The nap particle is an immunogenic surface adhesion complex from Mycoplasma genitalium. It is essential for motility and responsible for binding sialylated oligosaccharides on the surface of the host cell. Cryo-electron tomography (cryo-ET) of M. genitalium revealed the tetrameric organization of the nap particle complex, consisting of two P140-P110 heterodimers. The P140-P110 heterodimers form the ‘tight interface’, while the ‘loose interface’ is formed between the two heterodimers.

In contrast to previous studies, this analysis by classification of the native nap particle displayed both the ‘open’ and the ‘closed’ state of the tight interface, resolved at 17 Å and 18 Å, respectively. Although the resolution obtained is insufficient to resolve the sialylated oligosaccharides in the crown region, the fact that we obtain classes with the ‘open’ conformation is conclusive evidence for the bound state. The resulting structure of the P110-P140 interaction site in the crown region for the ‘open’ state shows that the distance between P110 and P140 at the tight interface is sufficiently large so that the interfering loop (P140 residues 807–827) no longer interferes with the β-hairpin of P110 (residues 455–465). The structure indicates that P140 may additionally stabilize the binding to sialylated oligosaccharides by forming hydrogen bonds with residues from region 631–634 and loop 870–877 of P140, such as those between residues N634, S871 and 6′-SL. The binding of 6′-SL is stabilized by hydrogen bonds from both P110 and P140. Importantly, the opening and closing of the tight interface is accompanied by an interaction between P110 and P140 at the loose interface of the nap particle. In the ‘closed’ conformation, there is no density seen at the loose interface, whereas in the ‘open’ conformation, P110 and P140 come into proximity at the loose interface, thus indicating an interaction between loop 662–666 of P110 and loop 1173–1179 of P140. In fact, classes showing an opening and closing of the tight interface are always associated with a repositioning of the P110 stalk. In the open state, nap particle is bound to sialylated oligosaccharides mediated by P110 and further stabilized by P140. In addition, there is an interaction between P110 and P140 at the loose interface.

> MKTMRKQIYKKAYWLLLPFLPLALANTFLVKEDSKNVTAYTPFATPITDSKSDLVSLAQLDSSYQIADQTIHNTNLFVLFKSRDVKVKYESSGSNNISFDSTSQGEKPSYVVEFTNSTNIGIKWTMVKKYQLDVPNVSSDMNQVLKNLILEQPLTKYTLNSSLAKEKGKTQREVHLGSGQANQWTSQRNQHDLNNNPSPNASTGFKLTTGNAYRKLSESWPIYEPIDGTKQGKGKDSSGWSSTEENEAKNDAPSVSGGGSSSGTFNKYLNTKQALESIGILFDDQTPRNVITQLYYASTSKLAVTNNHIVVMGNSFLPSMWYWVVERSAQENASNKPTWFANTNLDWGEDKQKQFVENQLGYKETTSTNSHNFHSKSFTQPAYLISGIDSVNDQIIFSGFKAGSVGYDSSSSSSSSSSSSTKDQALAWSTTTSLDSKTGYKDLVTNDTGLNGPINGSFSIQDTFSFVVPYSGNHTNNGTTGPIKTAYPVKKDQKSTVKINSLINATPLNSYGDEGIGVFDALGLNYNFKSNQERLPSRTDQIFVYGIVSPNELRSAKSSADSTGSDTKVNWSNTQSRYLPVPYNYSEGIIDADGFKRPENRGASVTTFSGLKSIAPDGFANSIANFSVGLKAGIDPNPVMSGKKANYGAVVLTRGGVVRLNFNPGNDSLLSTTDNNIAPISFSFTPFTAAESAVDLTTFKEVTYNQESGLWSYIFDSSLKPSHDGKQTPVTDNMGFSVITVSRTGIELNQDQATTTLDVAPSALAVQSGIQSTTQTLTGVLPLSEEFSAVIAKDSDQNKIDIYKNNNGLFEIDTQLSNSVATNNGGLAPSYTENRVDAWGKVEFADNSVLQARNLVDKTVDEIINTPEILNSFFRFTPAFEDQKATLVATKQSDTSLSVSPRIQFLDGNFYDLNSTIAGVPLNIGFPSRVFAGFAALPAWVIPVSVGSSVGILFILLVLGLGIGIPMYRVRKLQDASFVNVFKKVDTLTTAVGSVYKKIITQTGVVKKAPSALKAANPSVKKPAAFLKPPVQPPSKPEGEQKAVEVKSEETKS;> MHQPKKRLAKKSWAFLTAALTLGVITGVGGYFLFNQNKQRSSVSNFAYQPKQLSVKHQQAVDETLTPWTWNNNNFSSLKITGENPGSFGLVRSQNDNLNISSVTKNSSDDNLKYLNAVEKYLDGQQNFAIRRYDNNGRALYDINLAKMENPSTVQRGLNGEPIFDPFKGFGLTGNAPTDWNEIKGKVPVEVVQSPHSPNLYFVLLVPKVALEYHNLNNQVVKESLEVKATQSSFNPTQRLQKDSPVKDSSKQGEKLSETTASSMSSGMATSTRAKALKVEVERGSQSDSLLKNDFAKKPLKHKNSSGEVKLEAEKEFTEAWKPLLTTDQIAREKGMGATVVSFYDAPYSENHTAFGLVDHIDPKKMVENYPPSWKTPKWNHHGIWDYNARNLLLQTTGFFNPRRHPEWFDEGQAKADNTSPGFKVGDTDHKKDGFKKNSSSPIALPFEAYFANIGNMVAIGNSVFIFGGNGHATKMFTTNPLSIGVFRIKYTDNFSKSSVTGWPYAVLFGGLINPQTNGLKDLPLGTNRWFEYVPRMAVSGVKWVGNQLVLAGTLTMGDTATVPRLKYDQLEKHLNLVAQGQGLLREDLQIFTPYGWANRPDIPVGAWLQDEMGSKFGPHYFLNNPDIQDNVNNDTVEALISSYKNTDKLKHVYPYRYSGLYAWQLFNWSNKLTNTPLSANFVNENSYAPNSLFAAILNEDLLTGLSDKIFYGKENEFAENEADRFNQLLSLNPNPNTNWARYLNVVQRFTTGPNLDSSTFDQFLDFLPWIGNGKPFSNSPSPSTSASSSTPLPTFSNINVGVKSMITQHLNKENTRWVFIPNFSPDIWTGAGYRVQSANQKNGIPFEQVKPSNNSTPFDPNSDDNKVTPSGGSSKPTTYPALPNSISPTSDWINALTFTNKNNPQRNQLLLRSLLGTIPVLINKSGDSNDQFNKDSEQKWDKTETNEGNLPGFGEVNGLYNAALLHTYGFFGTNTNSTDPKIGFKADSSSSSSSTLVGSGLNWTSQDVGNLVVINDTSFGFQLGGWFITFTDFIRPRTGYLGITLSSLQDQTIIWADQPWTSFKGSYLDSDGTPKSLWDPTALKSLPNSSTTYDTNPTLSPSFQLYQPNKVKAYQTTNTYNKLIEPVDATSAATNMTSLLKLLTTKNIKAKLGKGTASSQGNNNGGGVSQTINTITTTGNISEGLKEETSIQAETLKKFFDSKQNNKSEIGIGDSTFTKMDGKLTGVVSTPLVNLINGQGATSDSDTEKISFKPGNQIDFNRLFTLPVTELFDPNTMFVYDQYVPLLVNLPSGFDQASIRLKVISYSVENQTLGVRLEFKDPQTQQFIPVLNASSTGPQTVFQPFNQWADYVLPLIVTVPIVVIILSVTLGLTIGIPMHRNKKALQAGFDLSNKKVDVLTKAVGSVFKEIINRTGISNAPKKLKQATPTKPTPKTPPKPPVKQ>QSNEAQTYYRNITEALKNPQNVRILNLSGSKLTTLPGEIGKLQNLQLLNLDDNQLIALPKEIGKLQNLQQLHLSKNQLMALPEEIGQLQNLQKLKLYENQLTAIPKEIGQLQNLQELNLAHNQLATLPEDIEQLQRLQTLYLGHNQFNSILKEIGQLQNLESLGLDHNQLNVLPKEIGQLRNLESLGLDHNQLNVLPKEIGQLQNLQILHLRNNQLTTLPKEIGQLQNLQKLLLNKNKLTTLPKEIGQLQNLQKLKLYENQLTTLPKEIGQ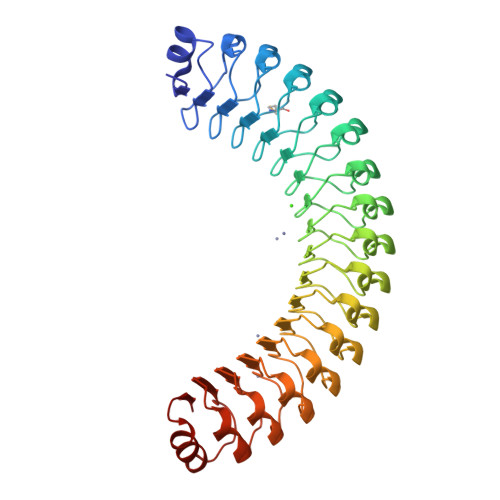LQNLQELDLDGNQLTTLPENIGQLQRLQTLYLGNNQLNFLPKEIGQLRNLESLDLEHNQLNALPKEIGKLQKLQTLNLKYNQLATLPEEIKQLKNLKKLYLHNNPLPSEKIARIRKLLPQCIIYFEE[2x]3-(3-methylphenyl)benzoic acid | C14 H12 O2 | 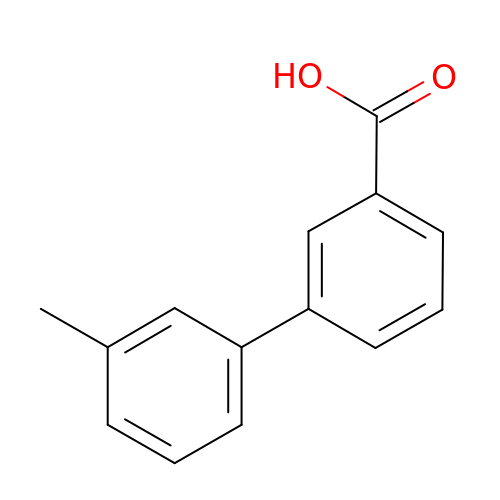BJVLFJADOVATRU-UHFFFAOYSA-N>[3x]MEMLTKFESRSSAAKGVAFHPTQPWILTSLHNGRIQLWDYRMGTLLDRFDGHDGPVRGIAFHPTQPLFVSGGDDYKVNVWNYKSRKLLFSLCGHMDYVRVCTFHHEYPWILSCSDDQTIRIWNWQSRNCIAILTGHSHYVMCAAFHPSEDLIVSASLDQTVRVWDISGLRMKNAAPVSMSKEDQKAQAHNSKSNDKKGSTD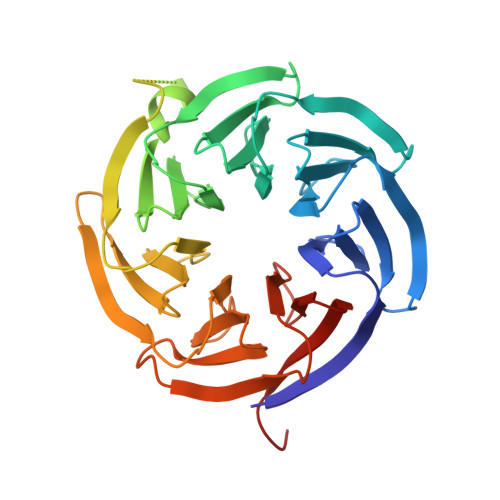AIVKFVLEGHDRGVNWCAFHPTLPLILSAGDDRLVKLWRMTASKAWEVDTCRGHFNNVSCCLFHPHQELILSASEDKTIRVWDLNRRTAVQTFRRDNDRFWFITVHPKLNLFAAAHDSGVMVFKLESAWSHPQFEK> MGSSKPLKGFVICCTSIDLKQRTEISTKATKLGAAYRSDFTKDVTHLIAGDFDTPKYKFAAKSRPDIKIMSSEWIPVLYESWVQGEDLDDGLLVDKHFLP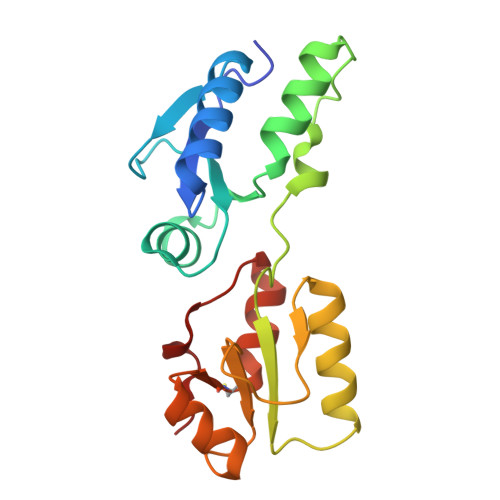TLFKCRVCLTNIGQPERSRIENYVLKHGGTFCPDLTRDVTHLIAGTSSGRKYEYALKWKINVVCVEWLWQSIQRNAVLEPQYFQLD> MGSSHHHHHHSSGLVPRGSHGSVLSNILVIAKDSSAASSATSGLNAYGIPYTTLLVPQAGVGLPALNSSNVGNYGGIVVAAEVSYDYGGTTGYQSALTTDQWNQLYAYQLEYGVRMVQFDVYPGPKFGASAVNGGCCNTGVEQLLSFTDTSDFPTAGLKTGATVSTEGLWHYPATISNSSNTKEIAQFAPNAVTSTASTAAVINNFDGREQMAFFIGFATDWSATSNYLQHAWITWLTRGLYAGHRRVNLNTQIDDMFLVTDIYYPNGSTFRITVEDMNGISAWVPTINAKMNPGSSYFVEVGHNGNGNIEQSSSTDAGAAACNGGGIEYDSPPDTPLEFKKPLGTGTDLWPSTPTTYDWTVACTQLDDLLRWWTTPANRDAFGHISHTFTHEEQNNATYADVFKEISFNQAWLKQVGLDQAKWFTSNGIIPPAITGLHNGDALQAWWDNGIRNCVGDNTRPVLMNQQNAMWPYFTTVESDGFAGMQVNPRWATRIYYNCDTPACTVQEWIDTSAGAGSFDDL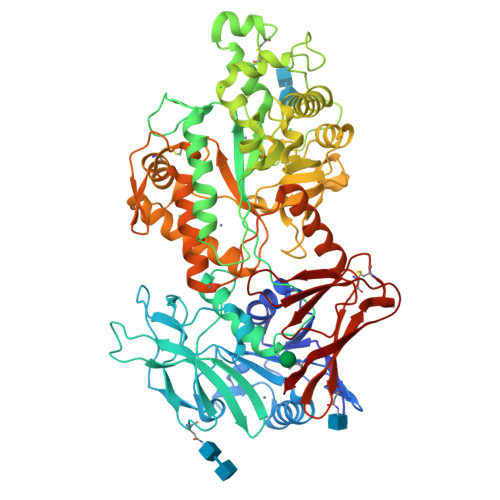LAVEKADTMRHLLGLRHDGYMFHQANLRNADVTPITVNGVTAKYSIFQAWVETIVQEFVRLVDWPLVTITHQEMSENFLARYQRDQCGYGLSYAVADKKITAVTVTATGNTCSRPIPVTFPVAPTSTQGYATEQLGSDPLTVWVQLSGSPVTFTLSTPIAL>GSHMFSLITWNIDGLDLNNLSERARGVCSYLALYSPDVIFLQEVIPPYYSYLKKRSSNYEIITGHEEGYFTAIMLKKSRVKLKSQEIIPFPSTKMMRNLLCVHVNVSGNELCLMTSHLESTRGHAAERMNQLKMVLKKMQEAPESATVIFAGDTNLRDREVTRSGGLPNNIVDVWEFLGKPKHCQYTWDTQMNSNLGITAACKLRFDRIFFRAAAEEGHIIPRSLDLLGLEKLDCGRFPSDHWGLLCNLDIIL[2x]

Tyrosyl-DNA phosphodiesterase 2 (TDP2) {also known as TRAF and TNF receptor-associated gene (TTRAP) or ETS1-associated protein II (EAPII) } is a 5′-tyrosyl DNA phosphodiesterase that can remove the covalently-attached abortive complexes generated by DNA topoisomerase II (TOP2) when it is unable to complete its normal catalytic cycle. Fortunately, this type of DNA lesion is efficiently repaired, in part though the action of TDP2, which hydrolyses the phosphotyrosyl bond in a magnesium cofactor-dependent reaction, leaving ligatable 5′-phosphate moieties. Consequently, TDP2 has attracted interest as a target for small molecule inhibitors that might have utility in overcoming innate or acquired resistance to TOP2 poisons. Using a ‘humanized’ mouse TDP2 expression construct, we have now determined X-ray crystal structures of the catalytic domain of TDP2 in complex with deazaflavin inhibitors, revealing the unusual molecular interactions underpinning their mode of action.

We obtained crystals of the catalytic domain of human TDP2 (hTDP2CAT–residues 113–362), in its unliganded form, using protein expressed in E. coli and purified using standard chromatographic procedures (see ‘Materials and Methods’). The expression construct contains a single-point mutant–C273S–which removes a potentially reactive surface cysteine, and that in our hands significantly improved the expression levels and solubility of the recombinant protein. However, crystals of hTDP2CAT typically diffracted both poorly and anisotropically. Through iterative screening of many crystals, we were eventually able to collect a dataset that could be truncated isotropically to a maximum resolution of 3.1 Å. The fold of the human protein is highly similar to that of mouse, worm, and zebrafish but with some important differences–see expanded description below.> MEKPLYTAEPVTLEDLQLLADLFYLPYEHGPKGAQMLREFQWLRANSSVVSVNCKGKDSEKIEEWRSRAAKFEEMCGLVMGMFTRLSNCANRTILYDMYSYVWDIKSIMSMVKSFVQWLGCRSHSSAQFLIGDQEPWA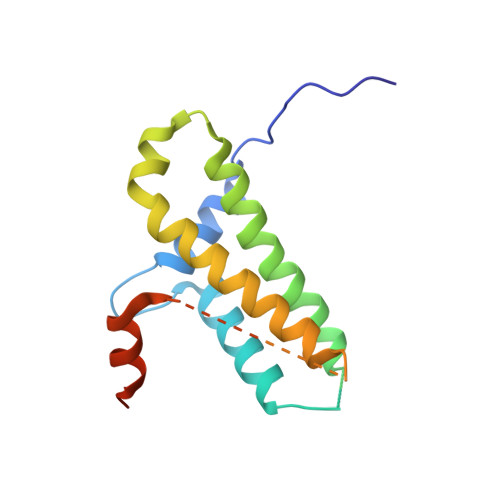FRGGLAGEFQRLLPIDGANDLFFQP> LAKPQNTAEVQKVQLTGEPVPMARCVSTGGRPPAQITWHSDLGGMPNTSQVPGFLS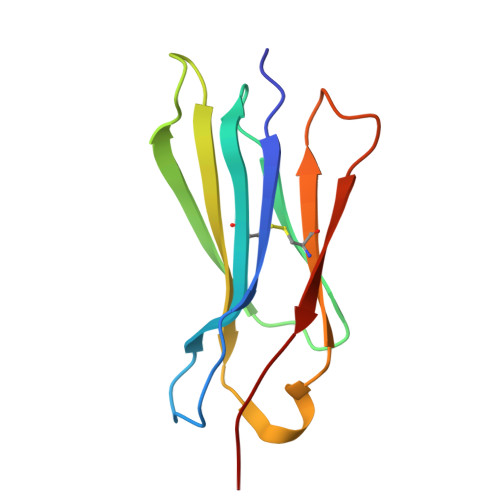GTVTVTSLWILVPSSQVDGKNVTCKVEHESFEKPQLLTVNLTVYYP> SMKRVQPCSLDPATQKLITNIFSKEMFKNTMALMDLDVKKMPLGKLSKQQIARGFEALEALEEALKGPTDGGQSLEELSSHFYTVIPHNFGHSQPPPINSPELLQAKKDMLLVLADIELAQALQAVSEQEKTVEEVPH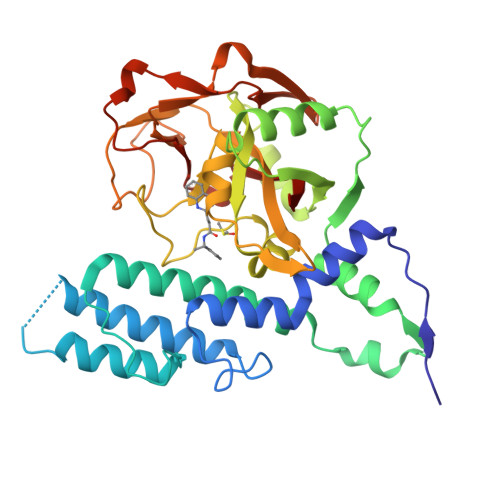PLDRDYQLLKCQLQLLDSGAPEYKVIQTYLEQTGSNHRCPTLQHIWKVNQEGEEDRFQAHSKLGNRKLLWHGTNMAVVAAILTSGLRIMPHSGGRVGKGIYFASENSKSAGYVIGMKCGAHHVGYMFLGEVALGREHHINTDNPSLKSPPPGFDSVIARGHTEPDPTQDTELELDGQQVVVPQGQPVPCPEFSSSTFSQSEYLIYQESQCRLRYLLEVH> GSSQLPQNIQFSPSAKLQEVLDYLTNSASLQMKSPAITATLEGKNRTLYMQSVTSIEERTRPNLSKTLKELGLVDGQELAVADVTTPQTV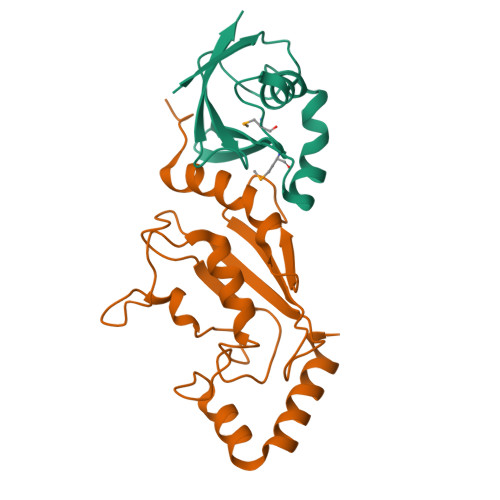LFKLHFTS;> GSATASDSTRRVSVRDKLLVKEVAELEANLPCTCKVHFPDPNKLHCFQLTVTPDEGYYQGGKFQFETEVPDAYNMVPPKVKCLTKIWHPNITETGEICLSLLREHSIDGTGWAPTRTLKDVVWGLNSLFTDLLNFDDPLNIEAAEHHLRDKEDFRNKVDDYIKRYAR> MRKGLWALVA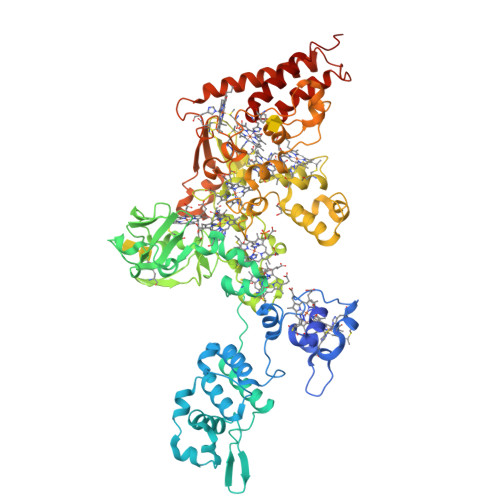AVLLLLVASPVLATEQYAKDTGKNCSYCHQVPASHKSQPGQQGRDQMDCMACHKAFMPLTSTAQIPLTERGVLFMQNGKKLAVDLNYDPLTEANVVKEFARVSGLSESAFGKVSGNITKQRLAYFLMVALKAQGEVAKVTANDLKKYADYTKAASANQKALVWAVKKGYLSARKAGSKLYLDPTAAASRTEVVKAFNAVQAKYPRVLPAPTAYAGTKKCQSCHGFSKFSATWHPNMVKTPDFFGSMLLWSLNDKFQASDVRYVINSPTELLFVGKDYKYMPYAFDKAENQWVADSHTQNWLVSCAKCHVTGYPGPNGITGTPYSVVGNTYKELFTEPGIGCEACHGPGALHAATGDPTKILGEKDGIAASATCEKCHEGAHHRGGEYNDEYAIAGVSGTVYGKHGISLQTIQKNSHGSVSCLECHSQDYRTALEDYLKANPGKTAADFNATVKLSDFKLGITCVTCHSPHSEKGYGKQLRKEPNELCMECHTGEGFTATSGSKGVHHPQKEVFTGQLGASFTALGIPEKVYNPMGSAECVTCHMPNGYHYFKVGKPTISIDNLTIKNDSSLGSYQSRYKASYNSCSVCHDAVGFDANAVKAWTDKVDTRVNNILNQLKTTYAAAYNDPNYKYADTLAGIVAADASHGIHNTALTELLLDKAEYYLTQIPKQ> KETAAAKFE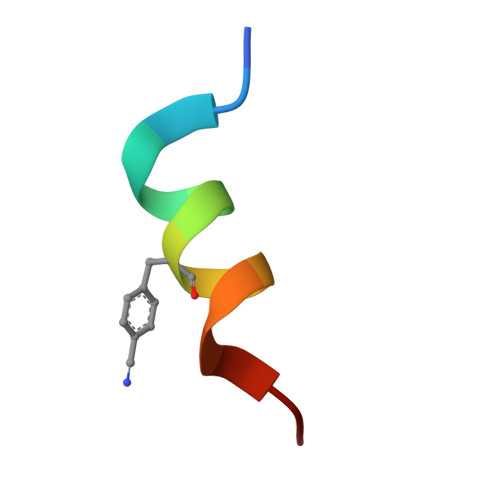RQHMDS> GSHMAIVKVTDADFDS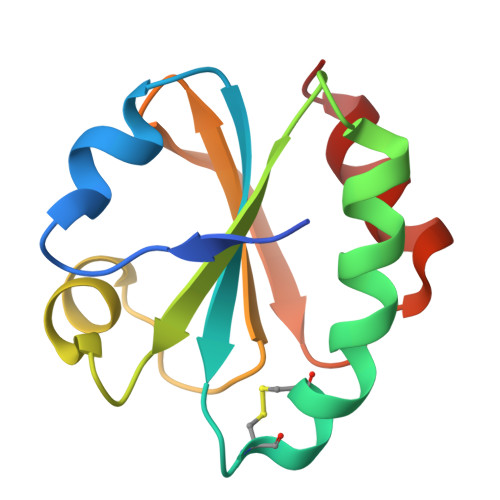KVESGVQLVDFWATWCGPCKMIAPVLEELAADYEGKADILKLDVDENPSTAAKYEVMSIPTLIVFKDGQPVDKVVGFQPKENLAEVLDKHL>[3x]MGSDKIHHHHHHMIQSYPVERSRTIQTRLVLPPDTNHLGTIFGGKVLAYIDEIAALTAMKHANSAVVTASIDSVDFKSSATVGDALELEGFVTHTGRTSMEVYVRVHSNNLLTGERTLT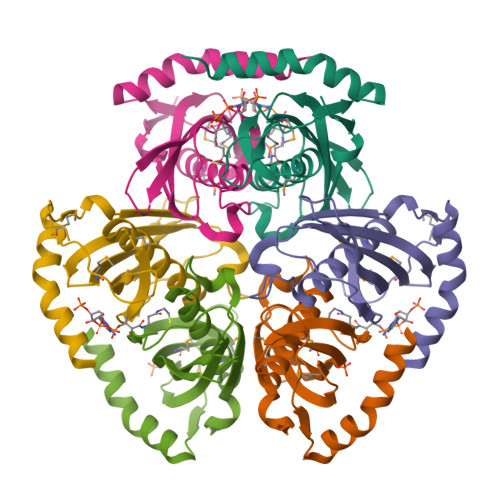TESFLTMVAVDESGKPKPVPQVEPQTEEEKRLYETAPARKENRKKRAALR N-{(1S)-1-[7-fluoro-2-(pyridin-2-yl)quinolin-3-yl]ethyl}-9H-purin-6-amine | C21 H16 F N7 | 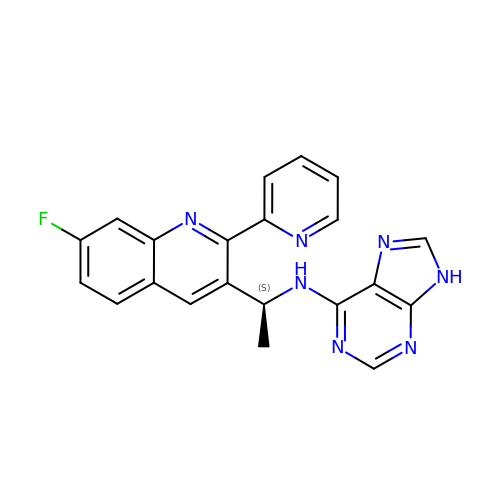KWRYMZHCQIOOEB-LBPRGKRZSA-N>SNAFDKLGNSAAIQEMNREVEAAAKRTSPVFLTGEAGSPFETVARYFHKNGTPWVSPARVEYLIDMPMELLQKAEGGVLYVGDIAQYSRNIQTGITFIIGKAERCRVRV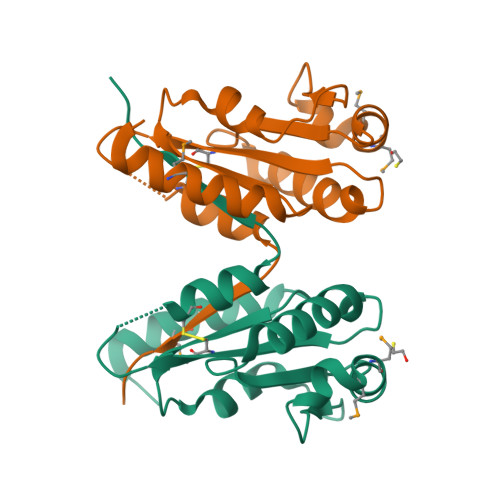IASCSYAAGSDGISCEEKLAGLFSESVVRIPPLS[2x]>[2x]FADDHAMSPDMKLLAGASNWVNQSGSVAQFVFTPSPTQPQTYEVSGNYINNAQG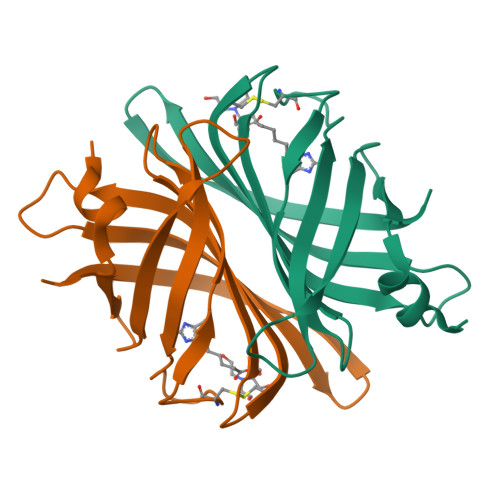TGCKGTPYPLSGAYYSGNQIISFSVVWSNASANCQSATGWTGYFDFSGSQAVLKTDWNLAFYSGSTPAIQQGQDDFMQSV> SMTGPIVYVQNADGIFFKLAEGKGTNDAVIHLANQDQGVRV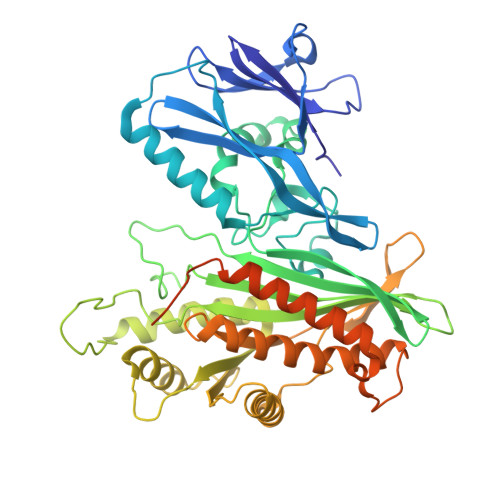LGAEEFPVQGEVVKIASLMGFIKLKLNRYAIIANTVEETGRFNGHVFYRVLQHSIVSTKFNSRIDSEEAEYIKLLELHLKNSTFYFSYTYDLTNSLQRNEKVGPAASWKTADERFFWNHYLTEDLRNFAHQDPRIDSFIQPVIYGYAKTVDAVLNATPIVLGLITRRSIFRAGTRYFRRGVDKDGNVGNFNETEQILLAENPESEKIHVFSFLQTRGSVPIYWAEINNLKYKPNLVLGENSLDATKKHFDQQKELYGDNYLVNLVNQKGHELPVKEGYESVVHALNDPKIHYVYFDFHHECRKMQWHRVKLLIDHLEKLGLSNEDFFHKVIDSNGNTVEIVNEQHSVVRTNCMDCLDRTNVVQSVLAQWVLQKEFESADVVATGSTWEDNAPLLTSYQNLWADNADAVSVAYSGTGALKTDFTRTGKRTRLGAFNDFLNSASRYYQNNWTDGPRQDSYDLFLGG>[2x]SKIFSKCELARKLKSMGMDGFHGYSLANWVCMAEYESNFNTQAFNGRNSNGSSDYGIFQLNSKWWCKS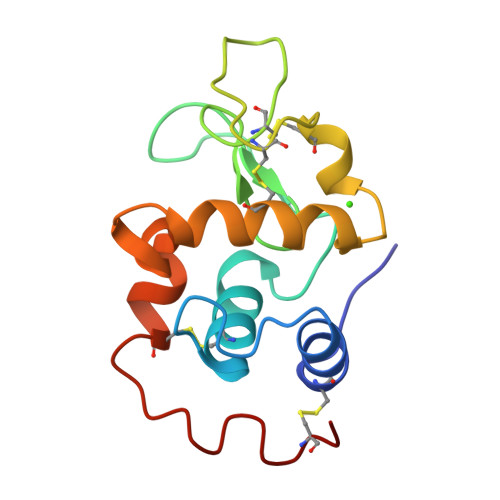NSHSSANACNIMCSKFLDDNIDDDIACAKRVVKDPNGMSAWVAWVKHCKGKDLSKYLASCNL>[2x]MKVAVLPGDGIGPEVTEAALKVLRALDEAEGLGLAYEVFPFGGAAIDAFGEPFPEPTRKGVEEAEAVLLGSVGGPKWDGLPRKIRPETGLLSLRKSQDLFANLRPAKVFPGLERLSPLKEEIARGVDVLIVRELTGGIYFGEPRGMSEAEAWNTERYSKPEVERVARVAFEFARKRRKHVVSVDKANVLEVGEFWRKTVEEVGRGYPDVALEHQYVDAMAMHLVRSPARFDVVVTGNI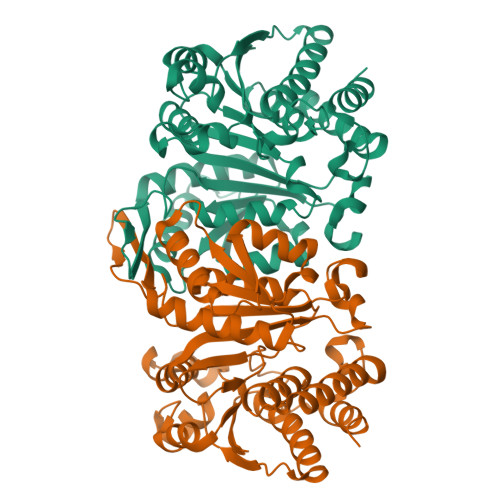FGDILSDLASVLPGSLGLLPSASLGRGTPVFEPVHGSAPDIAGKGIANPTAAILSAAMMLEHAFGLVELARKVEDAVAKALLETPPPDLGGSAGTEAFTATVLRHLA The bacterial member PspA is part of the phage shock protein (psp) response that maintains structural integrity of membranes under stress conditions such as temperature and infection. The main effector of the Psp system is PspA, a 25 kDa protein consisting of six α-helices connected by short loops and an elongated hairpin, where the N-terminal helix α0 of the protein remains unfolded in the absence of membranes. Interestingly, PspA is related to eukaryotic and archaeal endosomal sorting complexes required for transport (ESCRT)-III proteins and has a similar structure. Here, we show that rods of bacterial ESCRT-III protein PspA internalize and thin membrane tubules by overcoming the required bending energy through progressive membrane binding of the N-terminal helix in the PspA assembly.

Due to the critical role of helix α0 in membrane interaction, we also prepared and refolded an N-terminally truncated PspA including helices α1-5 in the presence of EPL liposomes. For the truncated PspA α1-5 sample, the total diameter distribution was narrower and ranged from 235 to 290 Å, with two maxima at 255 Å and 275 Å that were closer but not identical to the apo distribution of WT PspA. In the PspA α1-5 + EPL sample, we determined a total of five cryo-EM structures with resolutions ranging from 3.8 to 5.4 Å supported by visible side-chain details. For the α1-5 PspA variant, we found only five rod diameters (235, 250, 270, 280, and 290 Å), whereas two different symmetries (C1 and C2) could be identified for the diameter of 270 Å. None of these structures contained any additional lipid density in the rod lumen. Although the PspA mutant lacking helix α0 shows no structural alterations in the helical rod structure, it can no longer tubulate EPL membranes. In support of this analysis, when we abolished the α0–membrane interaction by removing helix α0 lacking this binding energy contribution, we did not observe any membrane internalization in the lumen of the PspA (α1-α5) rods in the cryo-EM images. Interestingly, when the protein was reconstituted in the presence of membranes, the ATPase activity was increased by ~210%, while the activity of PspA α1-5 was not affected in the presence of membranes.

>[60x]MGSSHHHHHHSSSAALEVLFQGPAPEDLLERLLGEMELELIELRRALAQTIATFKSTERQRDAQQLIAQRWYEKAQAALDRGNEQLAREALGQRQSYQSHTEALGKSLGEQRALVEQVRGQLQKLERKYLELKSQKNLYLARLKSAIAAQKIEEIAGNLDNASASSLFERIETKILELEAERELLNPPPSPLDKKFEQWEEQQAVEATLAAMKARRSLPPPSS GBS strains express either one of two SRR proteins, Srr1 or Srr2. We now report that both Srr1 and Srr2 bind to a specific tandem repeat region of fibrinogen Aα chain. As was previously predicted from sequence and functional analyses, Srr1-BR and Srr2-BR each adopt an overall fold that resembles the binding regions of “microbial surface components recognizing adhesive matrix molecules” (MSCRAMMs), including the well characterized ClfA, ClfB, SdrG, and the likely MSCRAMM UafA. Like other MSCRAMMs, Srr1-BR and Srr2-BR contain two domains, termed N2 and N3, with each adopting the DE variation of the Ig fold.

To assess whether Srr1 and Srr2 could support a DLL mechanism of ligand binding, we determined the crystal structures of S. agalactiae Srr1-BR and Srr2-BR at resolutions of 1.65 and 3.65 Å, respectively. An unusual feature of the Srr2-BR structure, not observed in Srr1-BR or in any previous structures of MSCRAMMs, is the conformation of the C terminus of the N3 domain. To date, the structures of MSCRAMMs crystallized in the absence of a ligand have the C-terminal extension of the N3 domain either completely or partially disordered. In contrast to other structurally characterized DLL proteins, the latch region in S. agalactiae Srr2-BR adopted a distinct conformation in the absence of ligand. Examination of the structures of the S. agalactiae Srr1 and Srr2 binding regions suggests how Srr2 might have greater affinity for the host ligand. In Srr2, the C-terminal latch of N3 appears to be pre-ordered in a conformation that might best be called “open, but ajar” that is poised to close over host ligand quickly. Although the cysteine cross-linking studies suggest that both Srr1 and Srr2 C termini are able to close even in the absence of ligand, the pre-ordered conformation of the C terminus in Srr2 would almost certainly require less time to do so. This would theoretically increase the kon and reduce the koff, and it could be numerically reflected as improved ligand affinity. To reveal whether the latch domain of Srr2-BR was important for binding, we generated a variant of the protein (Srr2-BRΔlatch), in which the terminal 13 residues of this domain were deleted. Removing the C-terminal amino acids of the Srr2 binding region abolished fibrinogen binding.

> METLPAALISGEGDVTTVQGQDVTDKLQNLDIKLSGGVQAKAGVINMDKSESMHMSLKFTIDSVNRGDTFEIKLSDNIDTNGASNYSIVEPIKSPTGEVYATGIYDSQKKSIVYSFTDFAASKNNINGILDIPLWPDDTTVQNTKEDVLFSVKIKDQEATIKETVKYDPPVRIDFAGGVSVDSRITNIDDVGKKMTYISQINVDGKSLYNYNGLYTRIYNYSKESTADLKNSTIKIYKTTSDNIVESMVQDYSSMEDVTSKFANSYPEKGWYDIYWGQFIASNETYVIVVETPFTNAVTLNTTLSDYNENNGVEHNHTYSSESGYSDVNAQERKILLEHHHHHH>[10x]DYKDDDDKLHSQANLMRLKSDLF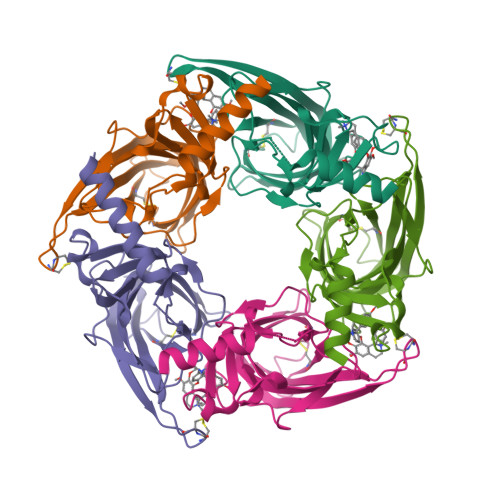NRSPMYPGPTKDDPLTVTLGFTLQDIVKADSSTNEVDLVYYEQQRWKLNSLMWDPNEYGNITDFRTSAADIWTPDITAYSSTRPVQVLSPQIAVVTHDGSVMFIPAQRLSFMCDPTGVDSEEGATCAVKFGSWVYSGFEIDLKTDTDQVDLSSYYASSKYEILSATQTRQVQHYSCCPEPYIDVNLVVKFRERRAGNGFFRNLFD>[3x]SMSRITIERDGLTLVGDREEPFGEIYDMAIIMHGFTANRNTDLLRQIADD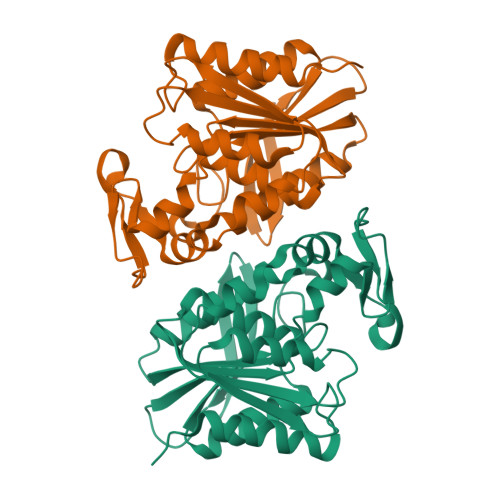LRDENVASVRFDFNGHGESDGKFEDMTVCNEIADGKAILDYVHTDPHVRDIFLVGHSQGGVVASMLAGLYPDVVKKVVLLAPAAQLKDDALRGNTQGATYDPNHIPDVVPLVGNKLGMKVGGFYLRTAQVLPIYEVSQRFTRPVSVIAGTNDQVVDPKYAKKYDEVYENSELHMIPNADHRFSGGYKDMAADLTAQFLKPAF> ASEEEKAWLMASRQQLAKETSNFGFSLLRKISMRHDGNMVFSPFGMSLAMTGLMLGATGPTETQIKRGLHLQALKPTKPGLLPSLFKGLRETLSRNLELGLTQGSFAFIHKDFDVKETFFNLSK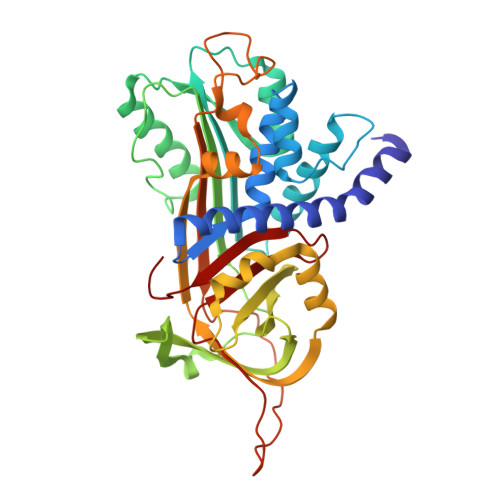RYFDTECVPMNFRNASQAKRLMNHYINKETRGKIPKLFDEINPETKLILVDYILFKGKWLTPFDPVFTEVDTFHLDKYKTIKVPMMYGAGKFASTFDKNFRCHVLKLPYQGNATMLVVLMEKMGDHLALEDYLTTDLVETWLRNMKTRNMEVFFPKFKLDQKYEMHELLRQMGIRRIFSPFADLSELSATGRNLQVSRVLQRTVIEVDERGTEAVAGILSEITAYSMPPVIKVDRPFHFMIYEETSGMLLFLGRVVNPTLL> MHHHHHHKNIVNTSILSIVYKKDDLIDLSRYGAKINIGDRVYYDSIDKNQIKLINLESSTIEVILKNAIVYNSMYENFSTSFWIKIPKYFSKINLNNEYTIINCIENNSGWKVSLNYGEIIWTLQDNKQNIQRVVFKYSQMVNISDYINRWMFVTITNNRLTKSKIYINGRLIDQKPISNLGNIHASNKIMFKLDGCRDPRRYIMIKYFNLFDKELNEKEIKDLYDSQSNPGILKDFWGNYLQYDKPYYMLNLFDPNKYVDVNNIGIRGYMYLKGPRGSVMTTNIYLNSTLYMGTKFIIKKYASGNEDNIVRNNDRVYINVVVKN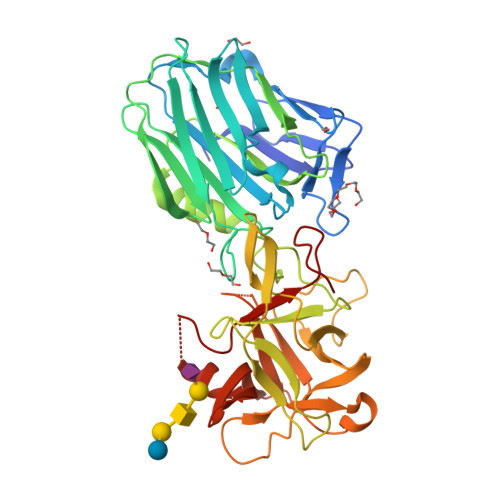KEYRLATNASQAGVEKILSALEIPDVGNLSQVVVMKSKDDQGIRNKCKMNLQDNNGNDIGFVGFHLYDNIAKLVASNWYNRQVGKASRTFGCSWEFIPVDDGWGESSL(4R,5S,6S,7R,9R,11E,13E,15S,16R)-16-ethyl-4-hydroxy-5,9,13,15-tetramethyl-2,10-dioxo-7-(2-oxoethyl)-1-oxacyclohexadeca-11,13-dien-6-yl 3,6-dideoxy-3-(dimethylamino)-beta-D-glucopyranoside 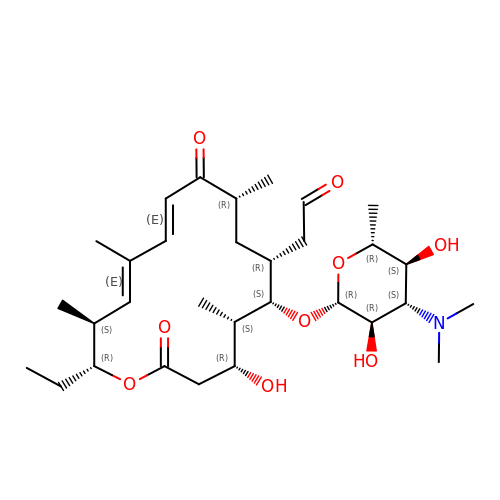| C31 H51 N O9 | FERSDKADYZRIAA-CQGKBTLCSA-N~{N}-[(1~{S})-1-(2-chloranyl-6-fluoranyl-phenyl)ethyl]-4-fluoranyl-1-[2-fluoranyl-5-(1-methylpyrazol-4-yl)phenyl]carbonyl-piperidine-4-carboxamide 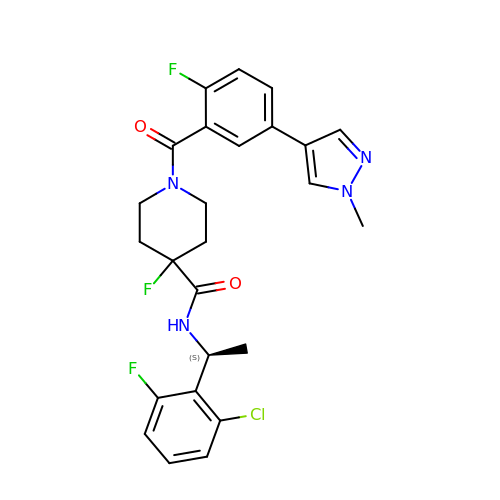| C25 H24 Cl F3 N4 O2 | HLEDGKCLFTZSGP-HNNXBMFYSA-N> GSQSTVDSIQSVLTTISSILSLKREKPDNLAIILQIDFTKLKEEDSLIVVYNSLKALTIKFARLQFCFVDRNNYVLDYGSVLHKIDSLDSISNLKSKSSSTQFSPIWLKNTLYPENI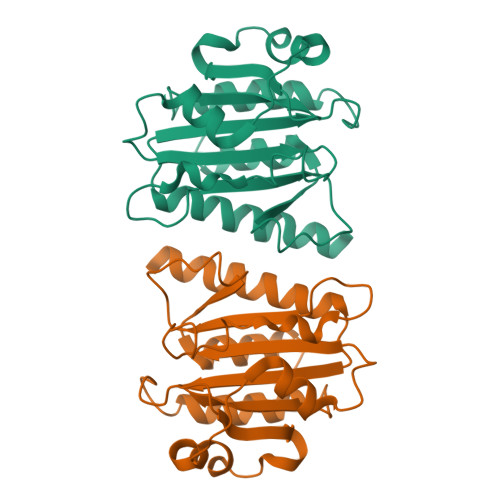HEHLGIVAVSNSNMEAKKSILFQDYRCFTSFGRRRPNELKIKVGYLNVDYSDKIDELVEASSWTFVLETLCYSFGLSFDEHDDDDEEDND> MAYWLMKSEPDEFSISDLQRLGKARWDGVRNYQARNFLRTMAEGDEFFFYHSSCPEPGIAGIGKIVKTAYPDPTALDPDSHYHDAKATTEKNPWSALDIGFVDIFKNVLGLGYLKQQSQLEQLPLVQKGSRLSVMPVTAEQWAAILALRLEHHHH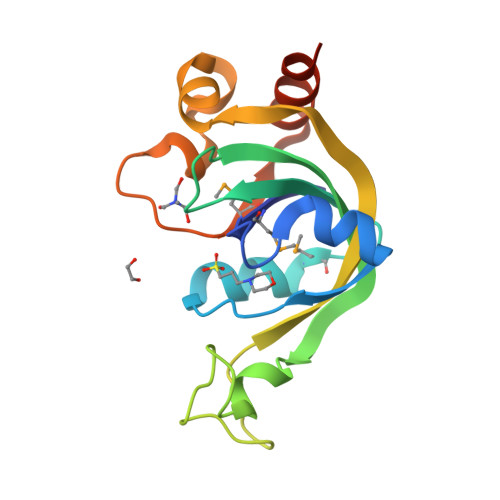HH The IALB_1185 protein, which is encoded in the gene cluster for endo-β-1,2-glucanase homologs in the genome of Ignavibacterium album, is a glycoside hydrolase family (GH) 35 protein. Here, we showed using recombinant IALB_1185 that this protein has glycosyltransferase activity toward β-1,2-glucooligosaccharides, and that the kinetic parameters for β-1,2-glucooligosaccharides are not within the ranges for general GH enzymes. Kinetic analysis further revealed that the enzyme has wide aglycone specificity regardless of the anomer, and that the β-1,2-linked glucose dimer sophorose is an appropriate donor. We propose that IALB_1185 be redefined β-1,2-glucooligosaccharide:d-glucoside β-d-glucosyltransferase as a systematic name and β-1,2-glucosyltransferase as an accepted name.

In order to understand the binding modes of ligands, the complex structures of WT with glucose (Glc) and Sop2 and the complex of the E343G mutant with 1-deoxynojirimycin (DNJ) were determined. When a crystal was soaked in a solution containing Glc, the electron densities of the Glc molecules were clearly observed in both subunits as the β-anomer at subsite +1 at almost the same positions as the DNJ molecule and the Glc moiety of Sop2. In contrast, Glc is absent at subsite −1 in the complex unlike in the DNJ and Sop2 complexes. If two Glc molecules bound at both subsites −1 and +1, the 1-hydroxy group (β-anomer) of a Glc molecule at subsite −1 and the 2-hydroxy group of a Glc molecule at subsite +1 would collide. These observations suggest that binding at subsite +1 is obviously stronger than that at subsite −1. In the WT-Glc complex, Arg349 participates in substrate recognition to give a stable conformation, whereas Glu102 is still disordered or flips out as the ligand-free structure. Subunit A of methyl-β-Glc, Sop2 and DNJ complexes, and both subunits of the Glc complex adopt the type 1 conformation, which is likely to be observed if the aglycone moiety of ligands is absent or small.

>SEKYFVKNGQPHFLISGEVHYFRINPKLWRNHLQLLKQTGADTVSTYIPWDWHEIEEDDFDFEGKTHPARNLIRFIKLCKEENLDLIVKPGPYILAEYENQGLPSWLLKKLSKNAFALDENGNVISPDLVSYLSDEFLEYTFKWYDKVMPIISKHQKEHYGPITMMQLCNEIGVFQWLSGKSDYNPKVINLYKEFIIQRYKTIEKLNSVYSTNYNSFDDLKAPSGKIKLRSDYCAYFDFHLFFREYYNKYISILKNKIRSFGINIKLTHNIPGWIYGNASELPMLISTYSEIMKNHPDIIFGLDHIPEFVSFRNAHSDLACNKILEAMQPEAPVWAAEFQAGTREHHVKAYAKDLETFYIASLAHGIKGFNYYMFSQGINPEGKGFYGKTFYFQTALDAASNKLALYDSIKKVNRFIRKEQKDLLRTNVNSEICVGFYKPYFFTELISSQLLKEKKLNVEELGLYIDPRFLREEILFNGLLRGLQTLNYNYDVVDLENCDLKSLTAYKQLWITSAEFMDAETQNLLSEFVLNGGNLILYPAVPTLDNYLNRCEILKNNFGIEFITKDSSHKVSAFGIEDVFTAFSKKQIYNDTNSKPIAFTQENEICGIRKKIGKGELTILGFAFGYTSDEHLELIDKLVKLNKIKRELFVSDKDIQFVVRENNKSRYIFFLNYHNERKTFNYRKSSELKKKKSEEISIAPFSYKVIKENK[2x]The cytochrome bc 1 complex, also known as respiratory complex III (CIII), in the electron-transfer chain of the inner mitochondrial membrane is a homodimer (CIII2) of two biochemically identical protomers. CIII2 catalyses the transfer of electrons from the lipophilic two-electron donor ubiquinol (QH2) to the water-soluble, one-electron acceptor protein cytochrome c, contributing to an electrochemical proton gradient across the membrane. Electron transfer within the complex occurs through the prosthetic groups of the three catalytic core subunits: heme b L and heme b H of cytochrome b (cyt b), heme c 1 of cytochrome c 1 (cyt c 1) and the [2Fe–2S] cluster of the iron–sulfur protein (ISP), often called the Rieske protein after its discoverer. The Rieske domain is tethered to the complex by one transmembrane helix and a connecting flexible linker that acts as a hinge.

The overall resolution of the consensus cryo-EM maps ranged from 2.1 to 3.3 Å for all samples. The consensus 3D refinement of combined particle images from all samples except the sample with atovaquone yielded a map with a resolution of 2.0 Å [Fig. 1(a)]. The three subunits of the catalytic core Cob (cyt b), Cyt1 (cyt c 1) and the transmembrane domain of Rip1 (ISP), as well as the seven supernumerary subunits of yeast CIII, Cor1, Qcr2, Qcr6–9 and the less tightly bound Qcr10, were well-resolved, consistent with other complete structures of CIII2 within respiratory supercomplexes from Saccharomyces cerevisiae. Density for the hydrophilic Rieske domains were equally poor in C1 and C2 refinements in all samples except that with atovaquone. Except for the sample with added Pf-type inhibitor, the Rieske domain map density was weak, as is commonly observed in uninhibited and hence unrestrained CIII2. Ten cardiolipin molecules on the matrix side, four molecules of DDM, four phosphocholines, four phosphatidylethanolamines and two phosphatidic acid molecules were modelled with truncated fatty-acid chains. We identified 1326 water molecules in the 2 Å resolution map of the dimeric complex.

>[2x]MNSLLRLPALKRGVFTMSKRGLATTVSPKTRTSNLKNGLTIASESNPLVQTATVGVWIDAGSRNENAYNNGTAHFFEHLAFKGTDKRSQHQLELDIENMGGHLNAYTSRESTVYYAKSFKDDVPKSVEILADILQHSKLAESAIDREREVITRELEEVNKQYEEVVFDHLHATAFMNQPLGRTILGPRENIQTITNTELRKFITENYTADRMVLVGAGAVDHDALVELAEKYFSHLPSSQSPVPLGTPRSSGEDANQNPIPNFVGSEVRLRDDTMPVAHIAIAVEGVSWTSEDYYTALVAQAIIGNYDRAVGTSRHQGSRLSNIVSENNLANSFQSFSTSYSDTGLWGIYLTSENTTQIDDLVHFTLKEWNRLSTSVSNLQVERAKSQLKAGLLLSLDGTTYVAEDIGRQLTTLGRRVTPAEVEAKLEAVTEHDVRAWAQKTLYDKDIALVGLGPIEGLYDYNRIRNDMSMMRW;>MTRGVPRLAVAARHFSTAEAAGVKVAAQDGQSPISDLSVVLRGGSRYATVPGVSHILEKFAFQNTVPKSALRFVRELELFGGKLYTHTTREHIVLRTQFLKQDLPYFVDAFANVLKETKFQQFELTERVAPVAELDLLKRESDPAFTALEAAHEVAFRTGLGNSVYAQGYSPVTLEDVKEFARQVYAKQNVAVVGNNVVPADLQQLVGTAFADLQEGSKVTQAGTTTLHGGEARVRTSTGNALTIALPIAEPKPVYHALASFLGGPASMPWSVGASPLAQATVGTHTSVKATYHNYGDAGLFAITIKGDSPAEISQVAHKAVQALKDTGAEVTEEQAARAYAKSKFAAAEAFENPDSSASVIGMELLSGVSRIAPENVQKFTPAELSEAAAQLSASAKPVVAAVGQVHALPFADELF[2x];>MALRKKNSLLNMANSYVLDSPQPSNLNYFWNFGSLLALCLVIQLATGITLAMHYTSHASLAFDSVEHIMRDVNFGWFIRYAHANTASFFFICIYAHMGRNIYYGSYKTPRVLPWSIGVIIFLLLIITAFMGYVLVFGQMSLWGATVICNLVSAIPWLGEDIVHFLWGGFSVGNPTLQRFFALHYLMPFVLAVFALLHLIALHTAGSSNPLGITSNVDKLSMHPYYSFKDLITVFAFLLMFTLFVFFSPDKLGHPDNYIPANPMVTPASIVPEWYLLPFYAILRAIPDKLGGVIAMVAAILILLILPIVDRSIIRGNAFKPISKLLFGFFICNFLLLGVLGQVHIEPPFIVLGQICTIFYFSYFLILLPMVSTIENIFFYIGSLRK[2x];>MRRRRIGVWPENRRVSRLWVSLSPRSCVTCPVPTNQNPPINNHHTPILTQMFKAIPLRQALLGISSAVCAGATTTYYYTTKAEAMTAAEHGLHPAEYPWPQNGMLSTFDHASLRRGYQVYKEVCAACHSLDRIAWRNLVGVTHTTDEAKAFAEELEYDDEPDDEGNPRKRPGKLADYIPGPYPNEQAARAANQGALPPDLSLIAKARHGGADYIFALLTGYPDEPPAGVVLAPGMNYNPYFPGGGIGMARTLFDGVVEYEDGTPATTSQMAKDVAAFLTWAAEPEHDERKKLGLKAIIVISAMLGLSVYIKKFKWSPIKNRKFIYNPPKN[2x];>[2x]MSLLRTAAQAVKAPKAYTPLVAAKAFAQTRSVSSQPIGGKSTYKIPDFTPYLKKDRNTDANRLFSYFMIGSFGMLSAAGAKATVQDFLSNMSASADVLAMAKVEVKLGAIPLGKNVIIKWRGKPIFIRHRTSEEIEEANEVNVATLRDPQTDDERVQKPEWLVMIGVCTHLGCVPIGEAGDFGGWFCPCHGSHYDISGRIRRGPAPLNLEIPEYDFADAETLVIG;>[2x]MSYFLTLASEVAESLLPTVAFASEEEKEQDEPVEVESDDDESEEKEDDDEEEDEDDDDDDDDDEVPDPAIALHEAAAEGPCHDFKHHFDECVERVTKAQEAEDYDHAEYKEDCVEEFFHLQHCINDNTADKLFRVLK;>[2x]MASITSVVKTSELILKSPLLSKIVVPLAKTYVKFSGYRQLGFKMNDLIIEETPNMQLALRRLPPTESYDRVYRLIRATQFSLSHKLATGNDITKPEEDDHYLIPYILDVEAEAFEKDALDNLEVVKRK;>MGGNGHYMGWWGHMGSPPQKGIAGYTISPFAARPFAGVVHAAIFNTFRRTKNQALFVILPVSFFYYVWTQASEKNEWLYTKAGRHELAKALAE[2x];>[2x]MAWATTFYNVFVKRNSAFVATILASAFVFDMTFETAIDNFWDRINAGKQWKDIRHKYIEAAGDDDEDDE;>[2x]MICGEGDYVKKPSYKIVPHFLGFNIPTVSKWIPIFGIWGAAAGIGALFLIEGVPRTRQDILSKIPIIGEHWIREIPASDNPF> MAKTYDYLFKLLLIGDSGVGKTCVLFRFSEDAFNSTFISTIGIDFKIRTIELDGKRIKLQIWDTAGQERFR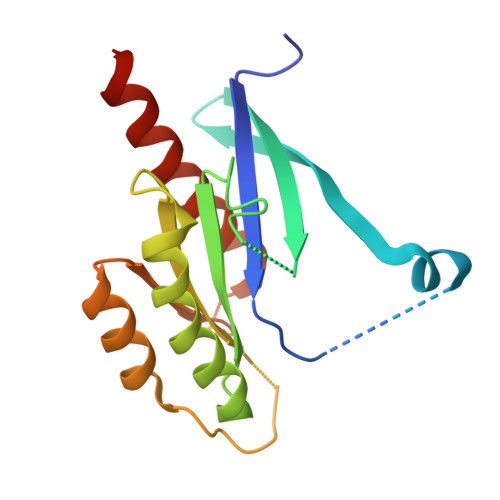TITTAYYRGAMGIMLVYDITNEKSFDNIRNWIRNIEEHASADVEKMILGNKCDVNDKRQVSKERGEKLALDYGIKFMETSAKANINVENAFFTLARDIKAKMDKNWKATAAG3-({4-[2-(3-chloroanilino)pyrimidin-4-yl]pyridin-2-yl}amino)propan-1-ol 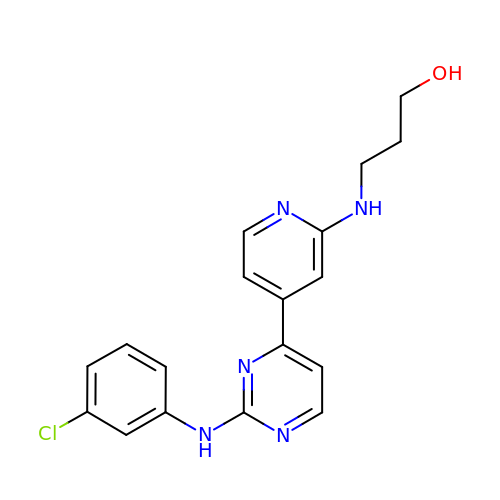| C18 H18 Cl N5 O | IYNDTACKOAXKBJ-UHFFFAOYSA-N> GPMTKSELIERIVTHQGQLSAKDVELAIKTMLEQMSQALATGDRIEIRGFGSFSLHYRAPRVGR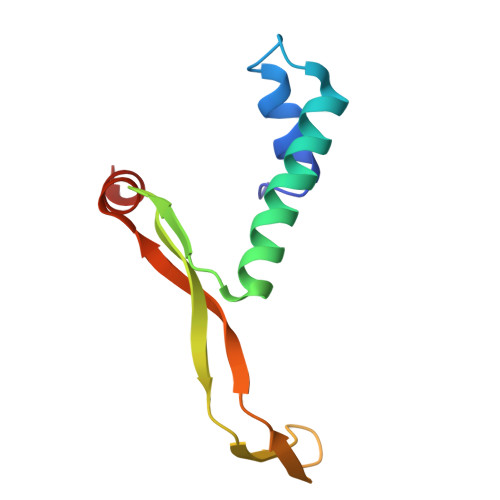NPKTGESVRLDGKFVPHFKPGKELRDRVNEPE> MSYLDNDYIGKNKDVGLKVELTEDIDRRIMEHRNRFRRLIFNRYVEFLPLLINYTNQNSVGIDFLQLEIALRQGYQVVVGKARNGVIMILGYIQSMYYKNS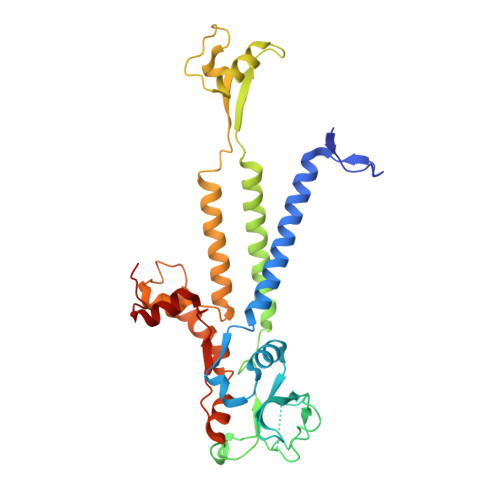NDFINNFNLTFNKRLTQDDITFIIPDYLRPDYALEIEYYDNCQSGDFIVLRNKPVNLNNDYQIIEHYCDELAEIILSRFSLIMQSKFSKIFLSDIQDETINQFINKLYNGAPFIKTDKYIDPEEDIIDLGSDFVTTALVEMKREYQNKVSELSNFLGVNSLAVDKESGVSDTEAKSNRSFTTSNSNIYLRGRNPFEMLNRRFNLDIHPYYDDEAISEMDIMNLKTDNFGGGKVE> MTVTRRHFLKLSAGAAVAGAFTGLGLSLAPTVARAELQKLQWAKQTTSICCYCAVGCGLIVHTAKDGQGRAVNVEGDPDHPINEGSLCPKGASIFQLGENDQRGTQPLYRAPFSDTWKPVTWDFALTEIAKRIKKTRDASFTEKNAAGDLVNRTEAIASFGSAAMDNEECWAYGNILRSLGLVYIEHQARIUHSPTVPALAESFGRGAMTNHWNDLANSDCILIMGSNAAENHPIAFKWVLRAKDKGATLIHVDPRFTRTSARCDVYAPIRSGADIPFLGGLIKYILDNKLYFTDYVREYTNASLIVGEKFSFKDGLFSGYDAANKKYDKSMWAFELDANGVPKRDPALKHPRCVINLLKKHYERYNLDKVAAITGTSKEQLQQVYKAYAATGKPDKAGTIMYAMGWTQHSVGVQNIRAMAMIQLLLGNIGVAGGGVNALRGESNVQGSTDQGLLAHIWPGYNPVPNSKAATLELYNAATPQSKDPMSVNWWQNRPKYVASYLKALYPDEEPAAAYDYLPRIDA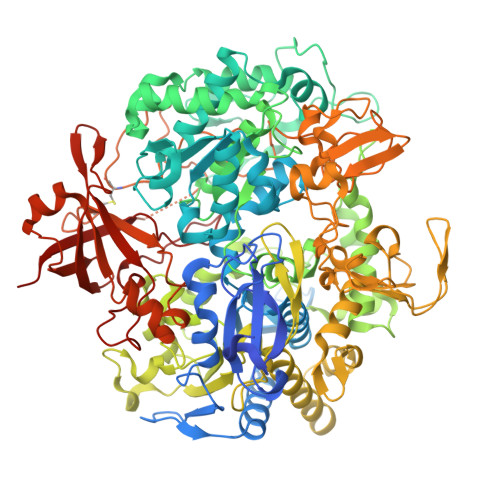GRKLTDYFWLNIFEKMDKGEFKGLFAWGMNPACGGANANKNRKAMGKLEWLVNVNLFENETSSFWKGPGMNPAEIGTEVFFLPCCVSIEKEGSVANSGRWMQWRYRGPKPYAETKPDGDIMLDMFKKVRELYAKEGGAYPAPIAKLNIADWEEHNEFSPTKVAKLMNGYFLKDTEVGGKQFKKGQQVPSFAFLTADGSTCSGNWLHAGSFTDAGNLMARRDKTQTPEQARIGLFPNWSFCWPVNRRILYNRASVDKTGKPWNPAKAVIEWKDGKWVGDVVDGGGDPGTKHPFIMQTHGFGALYGPGREEGPFPEHYEPLECPVSKNPFSKQLHNPVAFQIEGEKKAVCDPRYPFIGTTYRVTEHWQTGLMTRRCAWLVEAEPQIFCEISKELAKLRGIGNGDTVKVSSLRGALEAVAIVTERIRPFKIEGVDVHMVGLPWHYGWMVPKNGGDTANLLTPSAGDPNTGIPETKAFMVDVRKVWSHP> PNPCPESSASFLSRITFWWITGMMVQGYRQPLESTDLWSLNKEDTSEQVVPVLVKNWKKECAKSRKQPVKIVYSSKDPAKPKGSSKVDVNEEAEALIVKCPQKERDPSLFKVLYKTFGPYFLMSFLFKAVHDLMMFAGPEILKLLINFVNDKKAPEWQGYFYTALLFISACLQTLVLHQYFHICFVSGMRIKTAVIGAVYRKALVITNAARKSSTVGEIVNLMSVDAQRFMDLATYINMIWSAPLQVILALYLLWLNLGPSVLAGVAVMVLMVPLNAVMAMKTKTYQVAHMKSKDNRIKLMNEILNGIKVLKLYAWELAFKDKVLAIRQEELKVLKKSAYLAAVGTFTWVCTPFLVALSTFAVYVT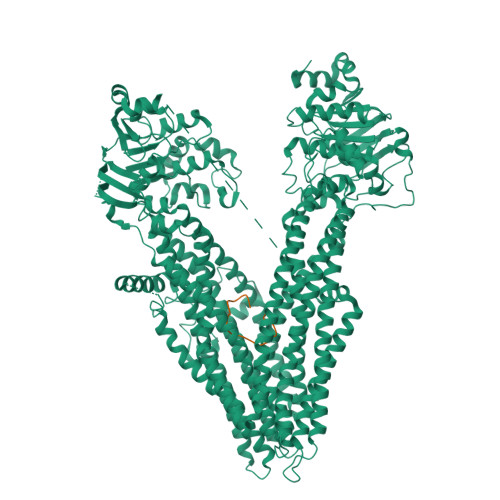VDENNILDAQKAFVSLALFNILRFPLNILPMVISSIVQASVSLKRLRVFLSHEDLDPDSIQRRPIKDAGATNSITVKNATFTWARNDPPTLHGITFSVPEGSLVAVVGQVGCGKSSLLSALLAEMDKVEGHVTVKGSVAYVPQQAWIQNISLRENILFGRQLQERYYKAVVEACALLPDLEILPSGDRTEIGEKGVNLSGGQKQRVSLARAVYCDSDVYLLDDPLSAVDAHVGKHIFENVIGPKGLLKNKTRLLVTHAISYLPQMDVIIVMSGGKISEMGSYQELLARDGAFAEFLRTYASAEQEQGQPEDGLAGVGGPGKEVKQMENGMLVTDTAGKQMQRQLSSSSSYSRDVSQHHTSTAELRKPGPTEETWKLVEADKAQTGQVKLSVYWDYMKAIGLFISFLSIFLFLCNHVASLVSNYWLSLWTDDPIVNGTQEHTQVRLSVYGALGISQGITVFGYSMAVSIGGIFASRRLHLDLLHNVLRSPISFFERTPSGNLVNRFSKELDTVDSMIPQVIKMFMGSLFNVIGACIIILLATPMAAVIIPPLGLIYFFVQRFYVASSRQLKRLESVSRSPVYSHFNETLLGVSVIRAFEEQERFIRQSDLKVDENQKAYYPSIVANRWLAVRLECVGNCIVLFASLFAVISRHSLSAGLVGLSVSYSLQVTTYLNWLVRMSSEMETNIVAVERLKEYSETEKEAPWQIQDMAPPKDWPQVGRVEFRDYGLRYREDLDLVLKHINVTIDGGEKVGIVGRTGAGKSSLTLGLFRIKESAEGEIIIDDINIAKIGLHDLRFKITIIPQDPVLFSGSLRMNLDPFSQYSDEEVWTSLELAHLKGFVSALPDKLNHECAEGGENLSVGQRQLVCLARALLRKTKILVLDEATAAVDLETDDLIQSTIRTQFDDCTVLTIAHRLNTIMDYTRVIVLDKGEIQEWGSPSDLLQQRGLFYSMAKDSGLV;> YFWGNLHWYYEQFDSTCX>[2x]SNAGGSATGTGLVYVDAFTRFHCLWDASHPECPARVSTVMEMLETEGLLGRCVQVEARAVTEDELLLVHTKEYVELMKSTQNMTEEE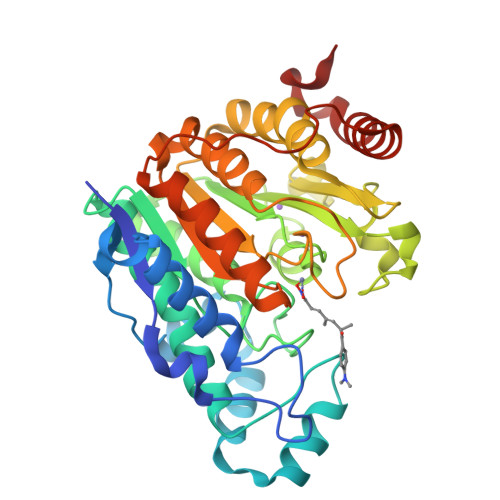LKTLAEKYDSVYLHPGFFSSACLSVGSVLQLVDKVMTSQLRNGFSINRPPGHHAQADKMNGFCMFNNLAIAARYAQKRHRVQRVLIVDWDVHHGQGIQYIFEEDPSVLYFSVHRYEDGSFWPHLKESDSSSVGSGAGQGYNINLPWNKVGMESGDYITAFQQLLLPVAYEFQPQLVLVAAGFDAVIGDPKGGMQVSPECFSILTHMLKGVAQGRLVLALEGGYNLQSTAEGVCASMRSLLGDPCPHLPSSGAPCESALKSISKTISDLYPFWKSLQTFE> GSHMELT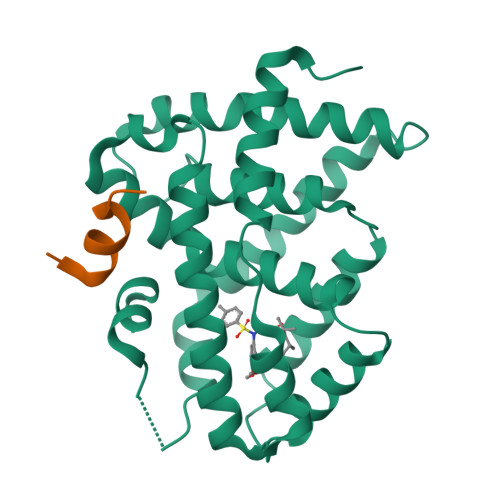PDQQTLLHFIMDSYNKQRMPQEITNKILKEAFSAEENFLILTEMATNHVQVLVEFTKKLPGFQTLDHEDQIALLKGSAVEAMFLRSAEIFNKKLPSGHSDLLEARIRNSGISDEYITPMFSFYKSIGELKMTQEEYALLTAIVILSPDRQYIKDREAVEKLQEPLLDVLQKLCKIHQPENPQHFACLLGRLTELRTFNHHHAEMLMSWRVNDHKFTPLLCEIWDVQ;> PSLLKKLLLAPA> ETG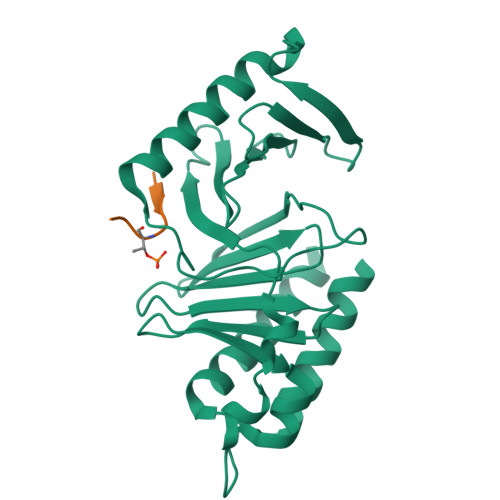EVVDCHLSDMLQQLHSVNASKPSERGLVRQEEAEDPACIPIFWVSKWVDYSDKYGLGYQLCDNSVGVLFNDSTRLILYNDGDSLQYIERDGTESYLTVSSHPNSLMKKITLLKYFRNYMSEHLLKAGANITPREGDELARLPYLRTWFRTRSAIILHLSNGSVQINFFQDHTKLILCPLMAAVTYIDEKRDFRTYRLSLLEEYGCCKELASRLRYARTMVDKLLSSRSASNRLKAS;> LLCSTPNGL> QPDGPLGPLFASSNPEYLSASDVFPSSVYVPDEWEVSREKITLLRELGQGSFGMVYEGNARDIIKGEAETRVAVKTVNESASLRERIEFLNEASVMKGFTCHHVVRLLGVVSKGQPTLVVMELMAHGDLKSYLRSLRPEAENNPGRPPPTLQEMIQMAAEIADGMAYLNAKKFVHRDLAARNCMVAHDFTVKIGDFGMTRDIYETDYYRKGGKGLLPVRWMAPESLKDGVFTTSSDMWSFGVVLWEITSLAEQPYQGLSNEQVLKFVMDGGYLDQPDNCPERVTDLMRMCWQFNPNMRPTFLEI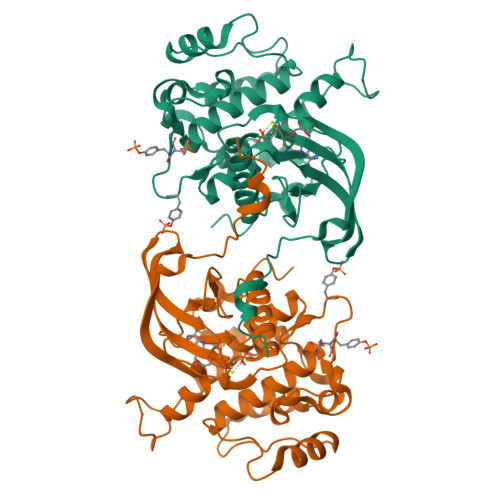VNLLKDDLHPSFPEVSFFHSEENK> GPGSTEKMEDVE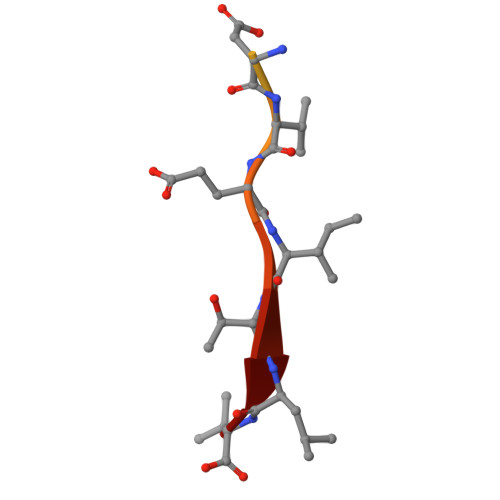ITLV> EASTTQNDTLKVMTHNVYML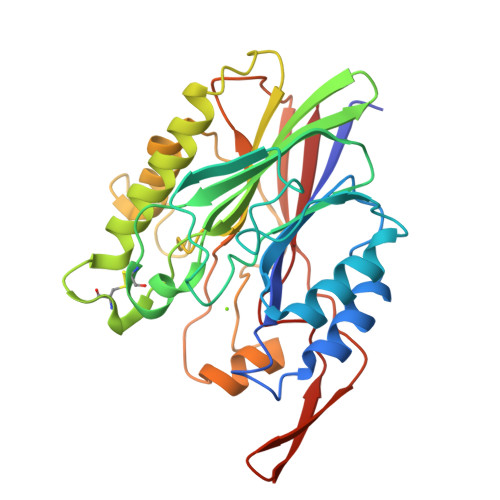STNLYPNWGQTERADLIGAADYIKNQDVVILNEVFDASASDRLLGNLKKEYPNQTAVLGRSSGSEWDKTLGNYSSSTPEDGGVAIVSKWPIAEKIQYVFAKGCGPDNLSNKGFVYTKIKKNDRFVHVIGTHLQAEDSMCGKTSPASVRTNQLKEIQDFIKNKNIPNNEYVLIGGDMNVNKINAENNNDSEYASMFKTLNASVPSYTGHTATWDATTNSIAKYNFPDSPAEYLDYIIASKDHANPSYIENKVLQPKSPQWTVTSWFQKYTYNDYSDHYPVEATISMK>MAHHHHHHMTTVRTRIAPSPTGDPHVGTAYIALFNLCFARQHGGQFILRIEDTDQLRSTRESEQQIYDALRWLGIEWDEGPDVGGPHGPYRQSERGHIYKKYSDELVEKGHAFTCFCTPERLDAVRAEQMARKETPRYDGHCMHLPKDEVQRRLAAGESHVTRMKVPTEGVCVVPDMLRGDVEIPWDRMDMQVLMKADGLPTYFLANVVDDHLMGITHVLRGEEWLPSAPKLIKLYEYFGWEQPQLCYMPLLRNPDKSKLSKRKNPTSITFYERMGYLPQALLNYLGRMGWSMPDEREKFTLAEMIEHFDLSRVS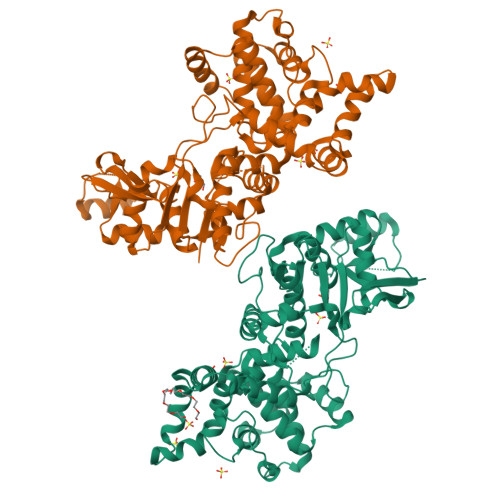LGGPIFDLEKLSWLNGQWIREQSVEEFAREVQKWALNPEYLMKIAPHVQGRVENFSQIAPLAGFFFSGGVPLDASLFEHKKLDPTQVRQVLQLVLWKLESLRQWEKERITGCIQAVAEHLQLKLRDVMPLMFPAITGHASSVSVLDAMEILGADLSRYRLRQALELLGGASKKETKEWEKIRDAIPG[2x]3-chloro-N-[(1R,2S)-2-phenylcyclopropyl]-5-{[(1H-pyrrolo[2,3-b]pyridin-5-yl)oxy]methyl}benzamide 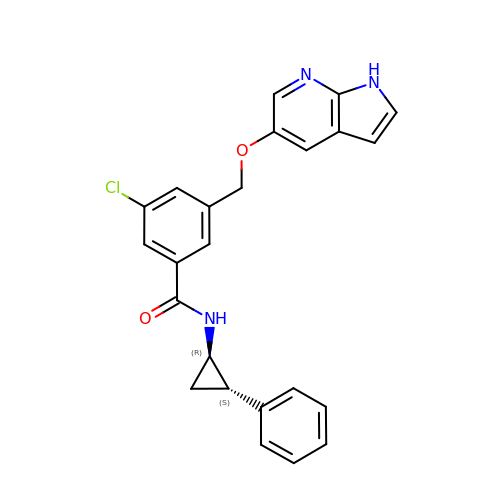| C24 H20 Cl N3 O2 | GICBMJSVILMECB-FCHUYYIVSA-N N-octyloctan-1-amine | C16 H35 N | 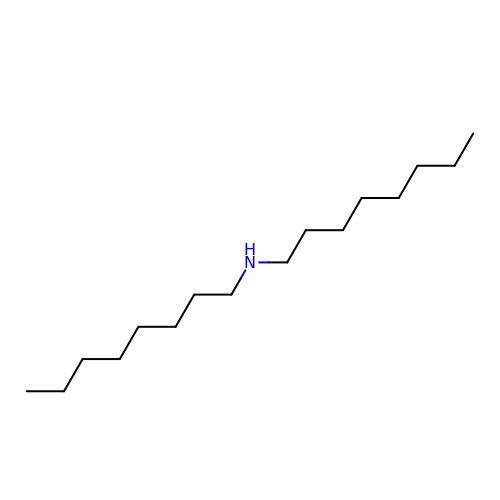LAWOZCWGWDVVSG-UHFFFAOYSA-N>[2x]MGSSHHHHHHSSGLGGTENLYFQSHMDE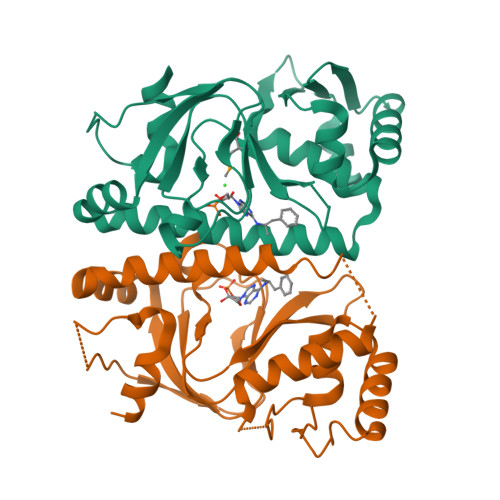ILARAGIFQGVEPSAIAALTKQLQPVDFPRGHTVFAEGEPGDRLYIIISGKVKIGRRAPDGRENLLTIMGPSDMFGELSIFDPGPRTSSATTITEVRAVSMDRDALRSWIADRPEISEQLLRVLARRLRRTNNNLADLIFTDVPGRVAKQLLQLAQRFGTQEGGALRVTHDLTQEEIAQLVGASRETVNKALADFAHRGWIRLEGKSVLISDSERLARRAR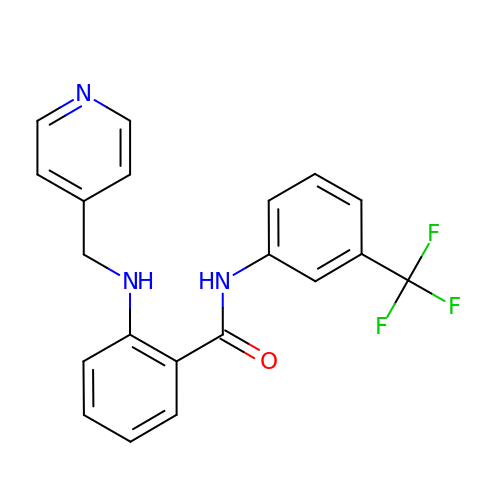2-(pyridin-4-ylmethylamino)-~{N}-[3-(trifluoromethyl)phenyl]benzamide | C20 H16 F3 N3 O | BLAFVGLBBOPRLP-UHFFFAOYSA-N>[4x]SLNTTGEPLTAFETFLPRVVMAEKIQDYQDSDAHEYMKAVQGYLDRFAVGDRLQNATRDLLVTFALAETGEKLSKRLPDQRVYMRDTFERHKDSADDRSAYLRHLRDTAAFIGNAWEPANNSPRALPGLEASAMTDTVKLCLAFLNSLKHTIAIAPLVRFYSEAVHADEGEAREKRVAE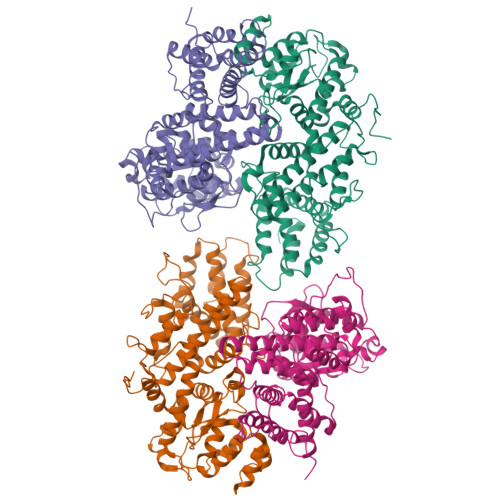FEKAIKAITAFTVFWRATRRGTGNIDSQYRAVMAGADSLTGIGPLARQWAEPDATKPDPDVDAEALKKELAARLSDPKGKGGVPNLASFLADASALPLYKISPPLARFLLLAAYHDTIEDPDNPGLIVQGKAGVASCFTADGWEDDTHLTIEHIAPQSATSGWDAEFYSDKETVHKLGNLVLAPGAANASLSSRPWTEKKVLYAALGASTADDAKSILNSSGFTFAQTTEDLAAMSRYLPHLRALGQREDELDPAFMDQRADVLLRLAYTRLKGWLGLELSDSSSDPVVKVDDVEVENGELDESGDAGAVVGTA>[3x]MSAIPCEGQNAEPASAASGEWQPRTPEQTLYAYVRCLNDSSASIEQKINWVKWHPDTTYESQCYVKCVSEELRLYDPKEKRFRPERFVLQAESFFHADPEQLQALKNNAEPMLAGVLADNSCESVFNKYATFYATHHSTILRMFHGDYRDIGNTYAKLGNGVKQIGQMFVDFCEKRTDFKWNEDNSCPPEAFLDCVFRGFRWITEEGEVNVNEIRRDYEAAGKGAADMADYCGSVKAGARQ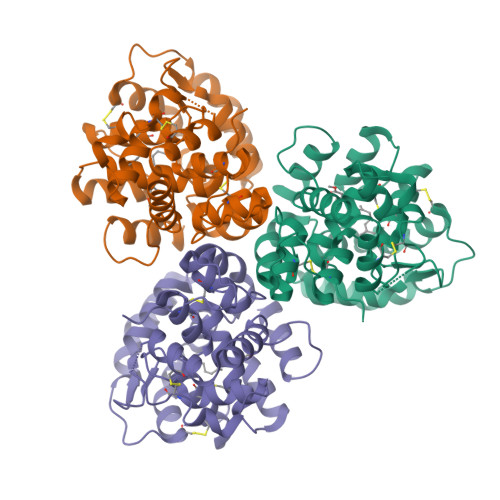LYNCLRDKGADSLVAVIRDRNQKTAFYFDLSSKEEPWKSAVDFANNL(4~{S})-6-azanyl-4-[3-cyano-5-[5-(methoxymethyl)thiophen-2-yl]phenyl]-3-methyl-4-propan-2-yl-2~{H}-pyrano[2,3-c]pyrazole-5-carbonitrile 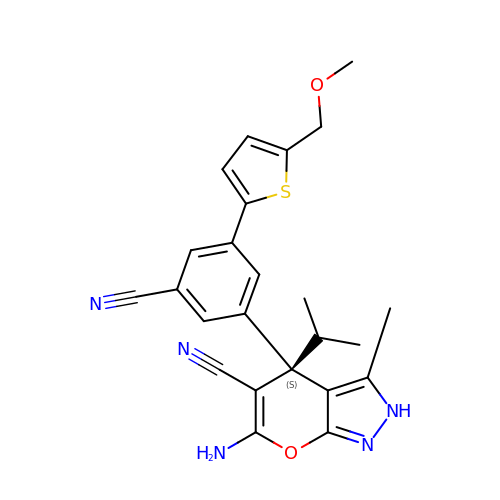| C24 H23 N5 O2 S | DRGJPMMQBOXCQB-DEOSSOPVSA-N>[2x]ETGQGQFSAGGCTFDDGPGACDYHQDLYDDFEWVHVSAQEPHYLPPEMPQGSYMIVDSSDHDPGEKARLQLPTMKENDTHCIDFSYLLYSQKGLNPGTLNILVRVNKGPLANPIWNVTGFTGRDWLRAELAVSTFWPNEYQVIFEAEVSGGRSGYIAIDDIQVLSYPCDKSPHFLRLGDVEVNAGQNATFQCIATGRDAVHNKLWLQRRNGEDIPVA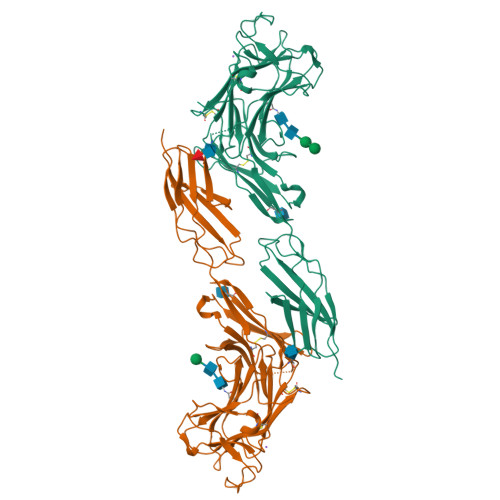QTKNINHRRFAASFRLQEVTKTDQDLYRCVTQSERGSGVSNFAQLIVREPPRPIAPPQLLGVGPTYLLIQLNANSIIGDGPIILKEVEYRMTSGSWTETHAVNAPTYKLWHLDPDTEYEIRVLLTRPGEGGTGLPGPPLITRTKGTKHHHHHH> MAHHHHHHMKPSLAKGTRDFTAQEVSRRKYIINTLQKNFELFGFQPLETPSFENLSTLTGKYGEEGDRLIFKILNSGNYTDKVNENDWQNKDAKKLTSQISDKALRYDLTVPFARFVAMNHGQLTFPFKRYQIQPVWRADRPQKGRFREFYQCDADVVGSESLWQEVELVQLYFKAFKELGVPVAIQMNNRKILSGLAE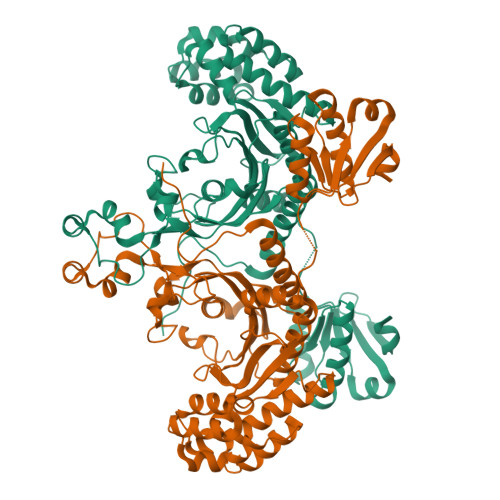YAGITEQLIDFTVALDKLDKIGKDGVIKEMQEKGISNEAIEKLDFLFHQKINALENLQELKTRFEGVEVGIQGVTELEFVLSKAMELGIDNQDLVFNITLARGLDYYTGAIFEVKAKGVEMGSIGGGGRYNNLTEVFGVKNIPGIGISFGLDRTYLVMEELGLFPENATVKVEYLFANYGEEEAIEAMKLIAQLREKGISAELYPEAAKLKKQFTYAEKKEIPNLVFLGKDEIENANVTIKNLTTGEQETITQSEFLK> MGSSHHHHHHSSGLVPRGSHSDEVDAHMMAEDMAAD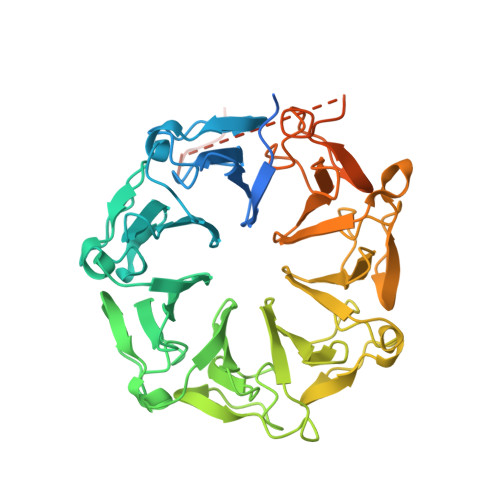EVTAPPRKVLIISAGASHSVALLSGDIVCSWGRGEDGQLGHGDAEDRPSPTQLSALDGHQIVSVTCGADHTVAYSQSGMEVYSWGWGDFGRLGHGNSSDLFTPLPIKALHGIRIKQIACGDSHCLAVTMEGEVQSWGRNQNGQLGLGDTEDSLVPQKIQAFEGIRIKMVAAGAEHTAAVTEDGDLYGWGWGRYGNLGLGDRTDRLVPERVTSTGGEKMSMVACGWRHTISVSYSGALYTYGWSKYGQLGHGDLEDHLIPHKLEALSNSFISQISGGWRHTMALTSDGKLYGWGWNKFGQVGVGNNLDQCSPVQVRFPDDQKVVQVSCGWRHTLAVTERNNVFAWGRGTNGQLGIGESVDRNFPKIIEALSVDGASGQHIESSNIDPSSGKSWVSPAERYAVVPDETGLTDGSSKGNGGDISVPQTDVKRVRI> MAAAAGRSLLLLLSSRGGGGGGAGGCGALTAGCFPGLGVSRHRQQQHHRTVHQRIASWQNLGA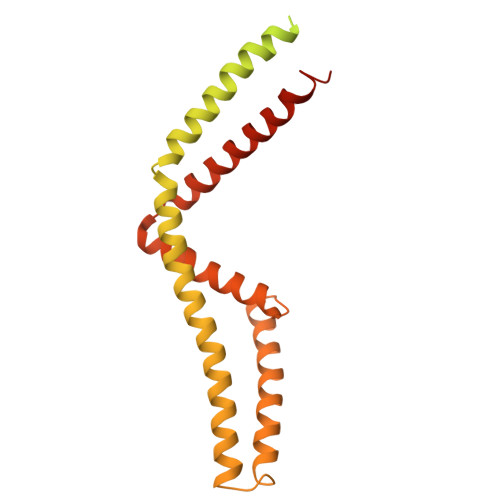VYCSTVVPSDDVTVVYQNGLPVISVRLPSRRERCQFTLKPISDSVGVFLRQLQEEDRGIDRVAIYSPDGVRVAASTGIDLLLLDDFKLVINDLTYHVRPPKRDLLSHENAATLNDVKTLVQQLYTTLCIEQHQLNKERELIERLEDLKEQLAPLEKVRIEISRKAEKRTTLVLWGGLAYMATQFGILARLTWWEYSWDIMEPVTYFITYGSAMAMYAYFVMTRQEYVYPEARDRQYLLFFHKGAKKSRFDLEKYNQLKDAIAQAEMDLKRLRDPLQVHLPLRQIGEKD>MNMAHTTTSMEIFGSPEQVWQLIGGFNSLPDWLPYIPSSKLTEGGRVRHLANPDGDTIIERLEVFNDKERYY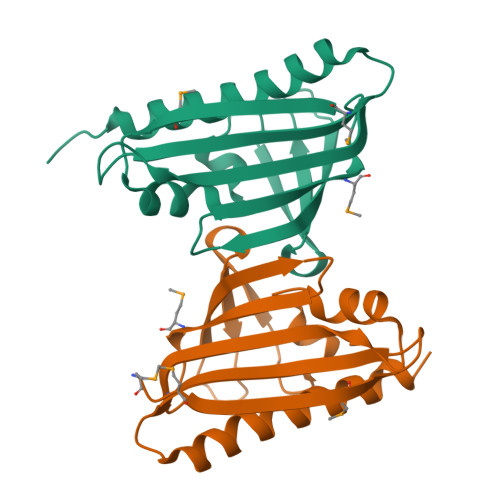TYSIMNAPFPVTNYLSTIQVKEGTESNTSLVEWSGTFTPVEVSDEEAINLFHGIYSDGLKALQQAFLDLEHHHHHH[2x]>[2x]MGTVMDVLKGDNRFSMLVAAIQSAGLTETLNREGVYTVFAPTNEAFRALPPRERSRLLGDAKELANILKYHIGDEI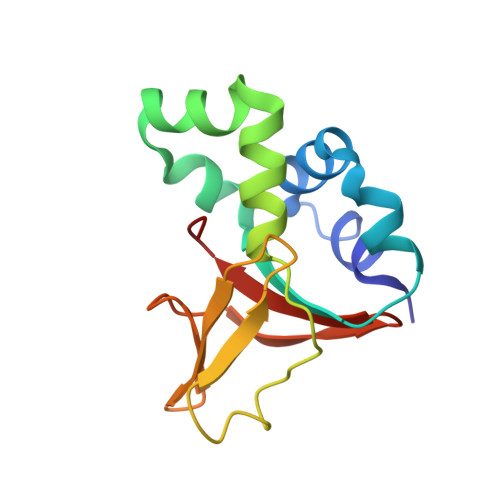LVSGGIGALVRLKSLQGDKLEVSLKNNVVSVNKEPVAEPDIMATNGVVHVITNVLQ>[2x]PSVYDAAAQLTADVKKDLRDSWKVIGSDK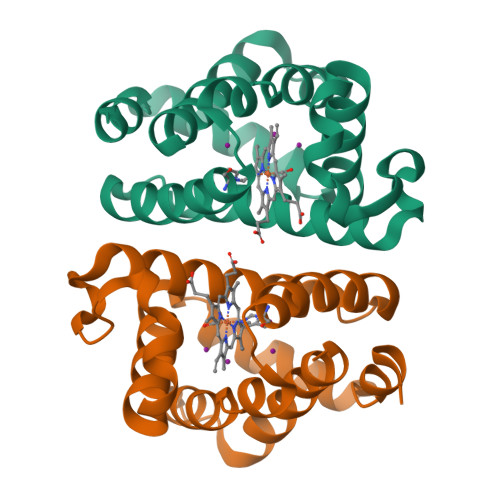KGNGVALMTTLFADNQETIGYFKRLGDVSQGMANDKLRGHSITLMYALQNFIDQLDNPDDLVCVVEKFAVNHITRKISAAEFGKINGPIKKVLASKNFGDKYANAWAKLVAVVQAAL>AQAPGRAPKAGSETIIAAAFSSLLGCDVQDADADFFALGGHXLLAMKLAAQLSRQVARQVTPGQVMVASTVAKLATIIDAEEDSTRRMGFETILPLREGNGPTLFCFHPASGFAWQFSVLSRYLDPQWSIIGIQSPRPNGPMQTAANLDEVCEAHLATLLEQQPHGPYYLLGYSLGGTLAQGIAARLRARGEQVAFLGLLDTWPPETQNWQEKEANGLDPEVLAEINREREAFLAAQQGSTSTELFTTIEGNYADAVRLLTTAHSVPFDGKATLFVAERTLQEGMSPERAWSPWIAELDIYRQDCAHVDIISPGTFE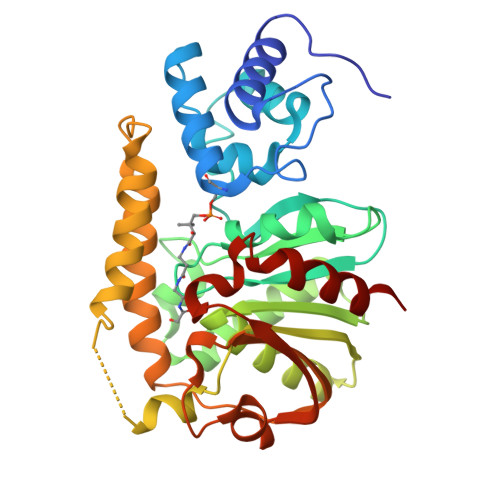KIGPIIRATLNR[2x]>GSMVAPSWRRPSRPEQRTEMYIDYDVSDRIATITLNRPEAANAQNPELLDELDAAWTRAAEDNDVSVIVLRANGKHFSAGHDLRGGGPVPDKLTLEFIYAHESRRYLEYSLRW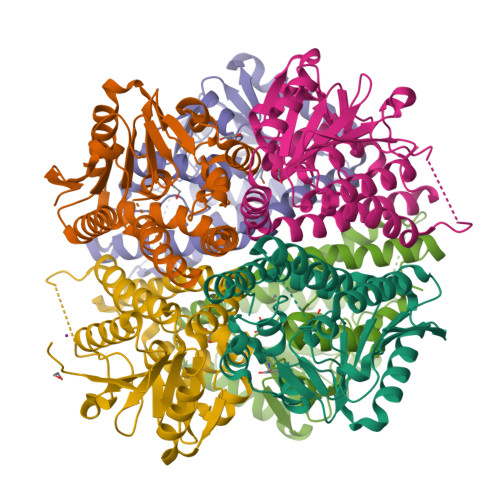RNVPKPSIAAVQGRCISGGLLLCWPCDLIIAAEDALFSDPVVLMDIGGVEYHGHTWELGPRKAKEILFTGRAMTAEEVAQTGMVNRVVPRDRLDAETRALAGEIAKMPPFALRQAKRAVNQTLDVQGFYAAIQSVFDIHQTGHGNAMSVSGWPVLVDIEEMKANIK[6x]>TTRDRVPTYQYNMNFEKLGKCIIINNKNFDKVTGMGVRNGTDKDAEALFKCFRSLGFDVIVYNDCSCAKMQDLLKKASEEDHTNAACFACILLSHGEENVIYGKDGVTPIKDLTAHFRGDRSKTLLEKPKLFFIQACRGTELDDGIQADSGPINDTDANPRYKAPVEADFLFAYSTVPGYYSWRSPGRGSWFVQALCSILEEHGKDLEIMQ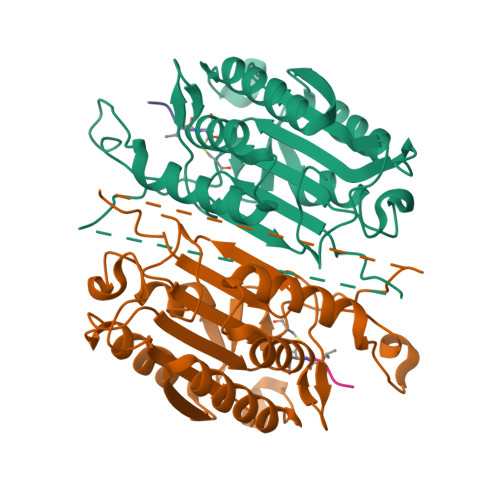ILTRVNDRVARHFESQSDDPHFHEKKQIPCVVSMLTKELYFSQHHHHHH[2x]> MHQGRLRLRPWLEEQIQSGRYPGVQWLDQSARVFQIPWKHAARHGWNIDKDATLFRNWAIHTGRYKPGIDKPDPKT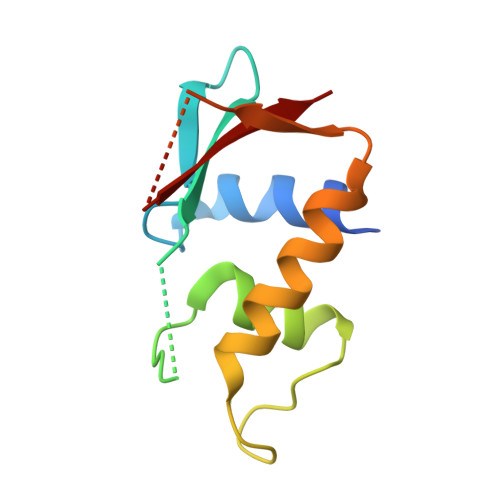WKANFRCALNSLTDVKELQDRSIKKGHNAFRVYALL> SGFVCNTCPEKWIN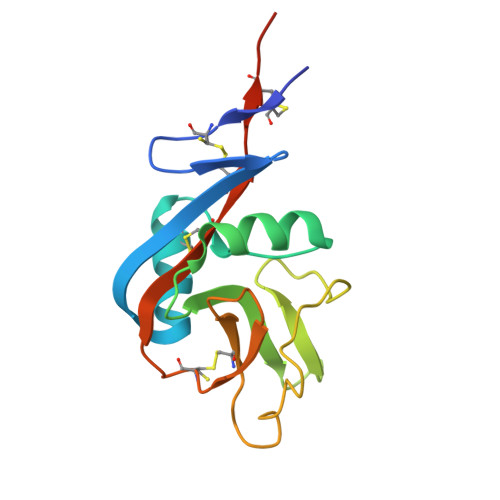FQRKCYYFGKGTKQWVHARYACDDMEGQLVSIHSPEEQDFLTKHASHTGSWIGLRDLDLEGEFIWVDGSHVDYSNWAPGEPNNRSQGEDCVMMRGSGRWNDAFCDRKLGAWVCDRLATCTPPASEGSAE> GIVIPPQEQITQHGSPYGRCANKTRALTVAELRGSGDLQEYLRHVTRGWSIFALYDGTYLGGEYGGVIKDGTPGGAFDLKTTFCIMTTRNTGQPATDHYYSNVTATRLLSSTNSRLCAVFVRSGQPVIGACTSPYDGKYWSMYSRLRKMLYLIYVAGISVRVHVSKEEQYYDYE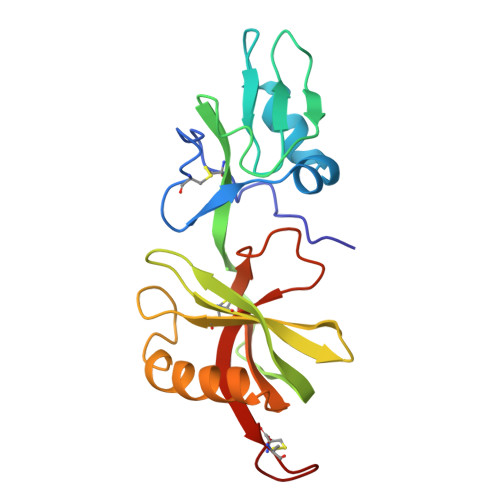DATFETYALTGISICNPGSSLC(3R,4S)-1-[6-(6-METHOXYPYRIDIN-3-YL)PYRIMIDIN-4-YL]-4-(2,4,5-TRIFLUOROPHENYL)PYRROLIDIN-3-AMINE 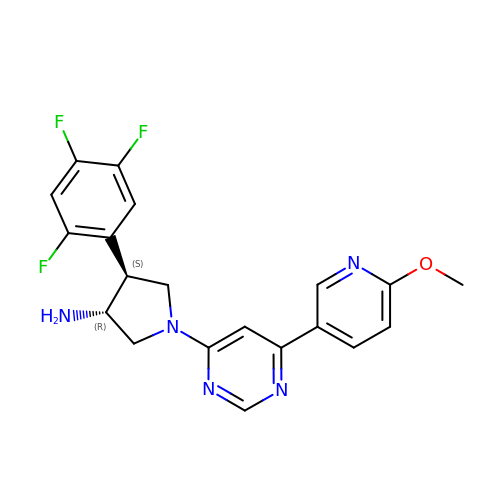| C20 H18 F3 N5 O | IFKWHPAWYJARQJ-DYVFJYSZSA-N> QKPGETKEVHPQLTTFRCTKRGGCKPATNFIVLDSLSHPIHRAEGLGPGGCGDWGNPPPKDVCPDVESCAKNCIMEGIPDYSQYGVTTNGTSLRLQHILPDGRVPSPRVYLLDKTKRRYEMLHLTGFEFTFDVDATKLPCGMNSALYLSEMHPTGAKSKYNPGGAYYGTGYCDAQCFVTPFINGLGNIEGKGSCCNAMDIWEANSRASHVAPHTCNKKGLYLCEGEECAFEGVCDKNGCGWNNYRVNVTDYYGRGEEFKVNTLKPFTVVTQFLANRRGKLEKIHRFYVQDGKVIESFYTNKEGVPYTNMIDDEFCEATGSRKYMELGATQGMGEALTRGMVLAMSIWWDQGGN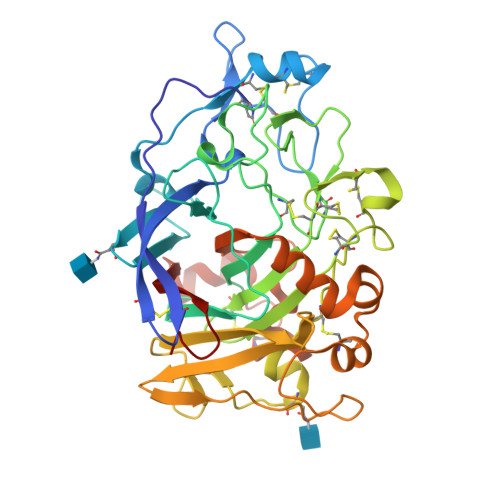MEWLDHGEAGPCAKGEGAPSNIVQVEPFPEVTYTNLRWGEIGSTYQELQ(4R)-4-{[(S)-tert-butoxy(hydroxy)methyl]amino}-5-[(1S)-cyclohex-2-en-1-ylselanyl]pentane-1,1-diol 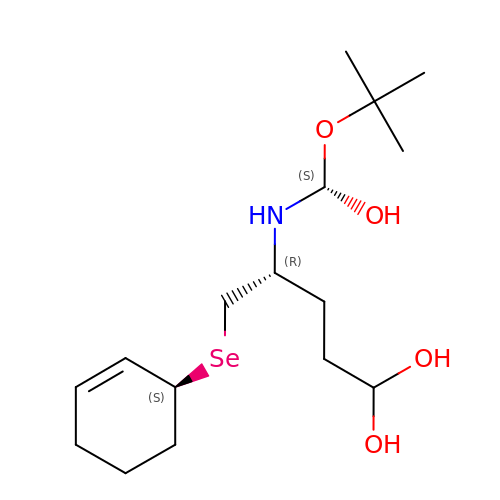| C16 H31 N O4 Se | UREOHWFKMYYNAM-NFAWXSAZSA-N> MENTENSVDSKSIKNLEPKIIHGSESMDSGISLDNSYKMDYPEMGLCIIINNKNFHKSTGMTSRSG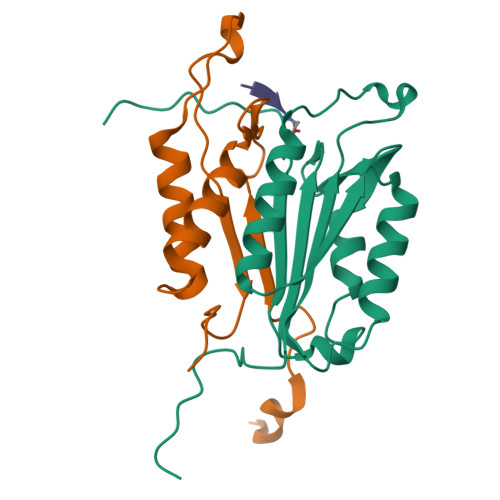TDVDAANLRETFRNLKYEVRNKNDLTREEIVELMRDVSKEDHSKRSSFVCVLLSHGEEGIIFGTNGPVDLKKITNFFRGDRCRSLVGKPKLFIIQACRGTELDCGIETD;> SGVDDDMACHKIPVEADFLYAYSTAPGYYSWRNSKDGSWFIQSLCAMLKQYADKLEFMHILTRVNRKVATEFESFSFDATFHAKKQIPCIVSMLTKELYFYHH>MAHHHHHHMALISMRQLLDHAAEHNYGVPAFNVNNLEQMRAIMLAADATNSPVIVQASAGARKYAGAPFLRHLILAAIEEWPHIPVVMHQDHGTSPDVCQRSIQLGFSSVMMDGSLGADGKTPTTYDYNVDVTRQVVAMAHACGVSVEGEIGCLGSLETGMAGEEDGVGAEGVLDHSQLLTSVEEAKQFVADTNVDALAIAVGTSHGAYKFTRPPTGDILAIDRIKEIHAALPNTHLVMHGSSSVPQEWLKVINEFGGNIGETYGVPVEQLVEAIKHGVRKIN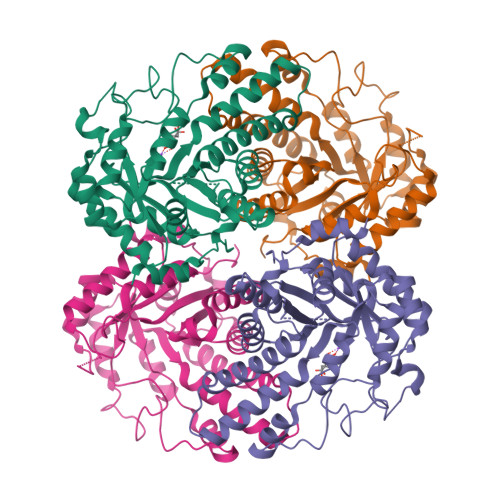IDTDLRLASTGAIRRFMAENPAEFDPRKYFAKTVDSMKQICIDRYEAFGTAGNADKIRPISLEKMVDRYK[2x]>[2x]DKIPNFVVPGKCASVDRNKLWAEQTPNRNSYAGVWYQFALTNNPYQLIEKCVRNEYSFDGKQFVIKSTGIAYDGNLLKRNGKLYPNP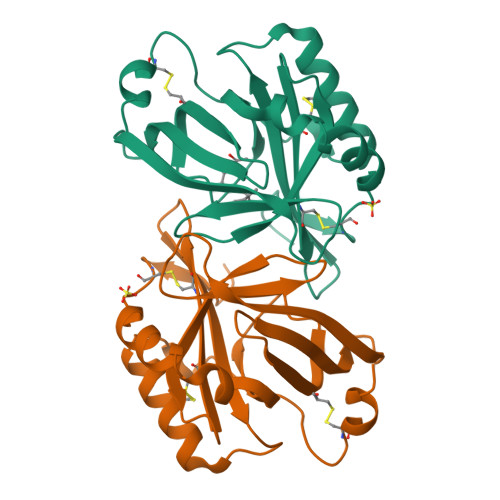FGEPHLSIDYENSFAAPLVILETDYSNYACLYSCIDYNFGYHSDFSFIFSRSANLADQYVKKCEAAFKNINVDTTRFVKTVQGSSCPYDTQKTL ABCB6 is an 842-amino acid protein that belongs to the B subfamily of the ABC transporter. ABCB6 is a “half-transporter” that contains a single pair of TMD and NBD, but needs to form a homodimer to be functional. ABCB6 is a porphyrin transporter located in the outer membrane of mitochondria that may regulate the heme biosynthetic pathway together with the plasma membrane porphyrin transporter ABCG216,17. ABCB6 plays a crucial role in energy-dependent porphyrin transport, drug resistance, toxic metal resistance, porphyrin biosynthesis, protection against stress, and encoding a blood group system Langereis antigen.

We solved the apo-state cryo-EM structure of human hABCB6 in nanodiscs at the resolution of 3.6 Å according to the Fourier shell correlation (FSC) 0.143 criterion. The hABCB6 apo-state structure shows an inward-facing conformation due to the absence of ATP. The overall structure shows an elongated shape with 130 Å in height and the two NBDs, like two “legs”, are separated by a distance of 35 Å. The TMD contains six transmembrane helices, among which TM4 and TM5 insert into the other hABCB6 monomer in the homodimeric transporter. In the apo-state, hABCB6 adopts an inward-facing conformation and TMDs of hABCB6 contain the substrate-binding cavity which is divided into two parts: a closed cavity 2 and an open-form cavity 1, different from the consecutive substrate-binding pocket found in most ABC transporters. The TMD region of hABCB6 contains a loop “plug”, just like a gate, which includes a sequence of “GGGTGSTG” in the middle region of TMD. The “plug” intervening TM2a and TM2b from one monomer interacts with TM5 and TM6 from another monomer of hABCB6, indicating that the “plug” is important for maintaining apo-form conformation and may undergo conformational changes during the transport process. The distance between those two “plugs” is about 6 Å and it is impassable for the substrates such as porphyrin. In the inward-facing conformation, the “plug” within the middle of the TMD region, and the upper constriction sites containing residues Y286 and V531, together forbid the access of substrate translocation. In the apo-state, the “plug” in TMD not only plays a role as a barrier to forbid the entry of substrates to cavity 2, but also maintains interactions with the neighboring monomer.

>MVTVGNYCEAEGPVGPAWMQDGLSPCFFFTLVPSTRMALGTLALVLALPCRRRERPAGADSLSWGAGPRISPYVLQLLLATLQAALPLAGLAGRVGTARGAPLPSYLLLASVLESLAGACGLWLLVVERSQARQRLAMGIWIKFRHSPGLLLLWTVAFAAENLALVSWNSPQWWWARADLGQQVQFSLWVLRYVVSGGLFVLGLWAPGLRPQSYTLQVHEEDQDVERSQVRSAAQQSTWRDFGRKLRLLSGYLWPRGSPALQLVVLICLGLMGLERALNVLVPIFYRNIVNLLTEKAPWNSLAWTVTSYVFLKFLQGGGTGSTGFVSNLRTFLWIRVQQFTSRRVELLIFSHLHELSLRWHLGRRTGEVLRIADRGTSSVTGLLSYLVFNVIPTLADIIIGIIYFSMFFNAWFGLIVFLCMSLYLTLTIVVTEWRTKFRRAMNTQENATRARAVDSLLNFETVKYYNAESYEVERYREAIIKYQGLEWKSSASLVLLNQTQNLVIGLGLLAGSLLCAYFVTEQKLQVGDYVLFGTYIIQLYMPLNWFGTYYRMIQTNFIDMENMFDLLKEETEVKDLPGAGPLRFQKGRIEFENVHFSYADGRETLQDVSFTVMPGQTLALVGPSGAGKSTILRLLFRFYDISSGCIRIDGQDISQVTQASLRSHIGVVPQDTVLFNDTIADNIRYGRVTAGNDEVEAAAQAAGIHDAIMAFPEGYRTQVGERGLKLSGGEKQRVAIARTILKAPGIILLDEATSALDTSNERAIQASLAKVCANRTTIVVAHRLSTVVNADQILVIKDGCIVERGRHEALLSRGGVYADMWQLQQGQEETSEDTKPQTMER[2x]> MAGVAEFNDKGELLLPKNYREWVMVGTQVTPNELNDGKAPFTEIRTVYVDPESYAHWKKTGEFRDGTVTVKELVSVGDRKGPGSGNGYFMGDYIGLEASVKDSQRFANEPGNWAFYIFYVPDTPLVAAAKNLPTAECAACHKENAKTDM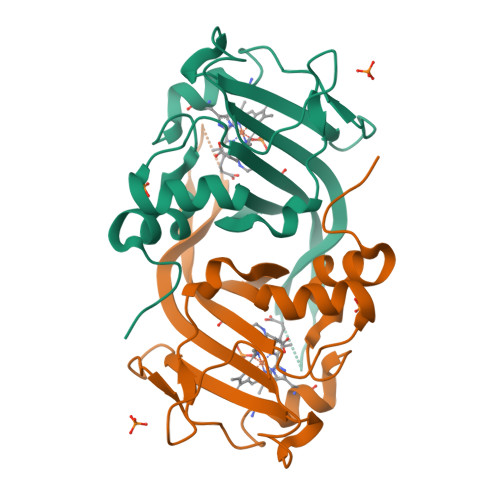VFTQFYPVLRAAKATGESGVVAPKKLAAALEHHHHHH>SMMSPNPLQKPAIDAAPAPFADFAPPVRPQSTLRRAITAAYRRPETECLPPLVEAATQSKEIRDAAASTARKLIEALRGKHSGSGVEGLVQEYSLSSQEGVALMCLAEALLRIPDTATRDALIRDKIADGNWKSHLGGSRSLFVNAATWGLVVTGKLTSTVNDRSLAAALTRLISRCGEPVIRRGVDMAMRMMGEQFVTGETIREALKRSKELEEKGFSYSYDMLGEAATTAADAERYYRDYESAIHAIGKASAGRGIYEGPGISIKLSALHPRYSRAQAARVMGELLPRVKALALLAKNYDIGLNIDAEEADRLELSLDLLEVLCLDGDLSGWNGMGFVVQAYGKRCPFVLDFIIDLARRSGRRIMVRLVKGAYWDAEIKRAQLDGLADFPVFTRKIHTDVSYIACAAKLLAATDVVFPQFATHNAQTLAAIYHMAGKDFHVGKYEFQCLHGMGEPLYEEVVGRGKLDRPCRIYAPVGTHETLLAYLVRRLLENGANSSFVHRINDPKVSIDELIADPVEVVRAMPVVGAKHDRIALPAELFGDARTNSAGLDLSNEETLASLTEALRESAAMKWTALPQLATGPAAGETRTVLNPGDHRDVVGSVTETSEEDARRAVRLAADAAPDWAAVPPSERAACLDRAAELMQARMPTLLGLIIREAGKSALNAIAEVREAIDFLRYYAEQTRRTLGPGHGPLGPIVCISPWNFPLAIFTGQIAAALVAGNPVLAKPAEETPLIAAEGVRILREAGIPASALQLLPGDGRVGAALVAAAETAGVMFTGSTEVARLIQAQLADRLSPAGRPIPLIAETGGQNAMIVDSSALAEQVVGDVITSAFDSAGQRCSALRVLCLQEDVADRILTMLKGALHELHIGRTDRLSVDVGPVITSEAKDNIEKHIERMRGLGRKVEQIGLASETGVGTFVPPTIIELEKLSDLQREVFGPVLHVIRYRRDDLDRLVDDVNATGYGLTFGLHTRLDETIAHVTSRIKAGNLYINRNIIGAVVGVQPFGGRGLSGTGPKAGGPLYLGRLVTTAPVPPQHSSVHTDPVLLDFAKWLDGKGARAEAEAARNAGSSSALGLDLELPGPVGERNLYTLHARGRILLVPATESGLYHQLAAALATGNSVAIDAASGLQASLKNLPQTVGLRVSWSKDWAADGPFAGALVEGDAERIRAVNKAIAALPGPLLLVQAASSGEIARNPDAYCLNWLVEEVSASINTAAAGGNASLMAIG[2x]

The proline catabolic pathway consisting of proline dehydrogenase (PRODH) and L-glutamate-γ-semialdehyde (GSAL) dehydrogenase (GSALDH) catalyzes the four-electron oxidation of L-proline to L-glutamate. PRODH is a flavoenzyme that catalyzes the FAD-dependent oxidation of L-proline to Δ1-pyrroline-5-carboxylate (P5C). Also known as ALDH4A1, GSALDH is a member of the aldehyde dehydrogenase (ALDH) superfamily and catalyzes the NAD+-dependent oxidation of GSAL to L-glutamate. In contrast, in some bacteria, most notably Gram-negative bacteria, the PRODH and GSALDH genes are combined into the putA gene, which encodes a bifunctional enzyme, proline utilization A (PutA).

Fragments 7 and 13 were bound to the GSAL substrate-binding site of the GSALDH active site. The refined occupancies of 7 were 0.83 and 0.86 in chains A and B of the asymmetric unit, respectively. Fragments 7 and 13 engaged well-known recognition elements of ALDH superfamily enzyme active sites. The carboxylates formed hydrogen bonds with the backbone of the anchor loop (1000s loop in SmPutA). The carboxylates also formed an ion pair with Arg843 and a hydrogen bond with Ser845. The heterocycles were flanked by two Phe side chains, which formed the so-called aromatic box of ALDH active sites. The dioxane ring of 7 forms a hydrogen bond with Arg843. The cyclic structures of 7 and 13 were perpendicular to the side chain of the glutamate product and, thus, could not access the oxyanion hole. The most notable inhibition occurred with 7 and 13, whose poses and interactions mimicked the substrate GSAL. The data were fitted to a global competitive inhibition model, resulting in Ki values of 0.32 mM ± 0.02 mM for 7 and 1.5 mM ± 0.1 mM for 13.>NTTQQGSPVFAKLLAKNQA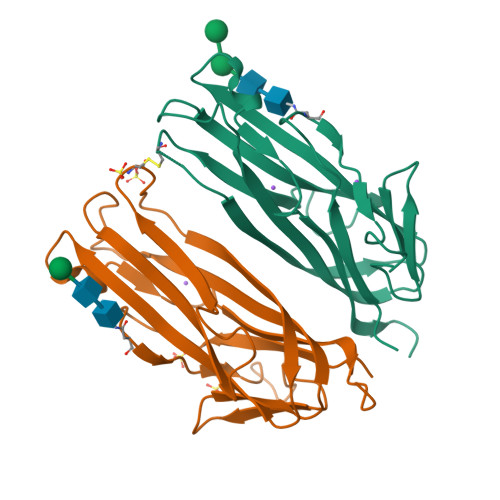SLCNTTLNWHSQDGAGSSYLSQGLRYEEDKKELVVDSPGLYYVFLELKLSPTFTNTGHKVQGWVSLVLQAKPQVDDFDNLALTVELFPCSMENKLVDRSWSQLLLLKAGHRLSVGLRAYLHGAQDAYRDWELSYPNTTSFGLFLVKPDNPWE[4x]> MAASRANDAPIVLLHGFTGWGREEMFGFKYWGGVRGDIEQWLNDNGYRTYTLAVGPLSSNWDRACEAYAQLVGGTVDYGAAHAAKHGHARFGRTYLGLLPELKRGGRIHIIAHSQGGQTARMLVSLLENGSQEEREYAKAHNVSLSPLFEGGHHFVLS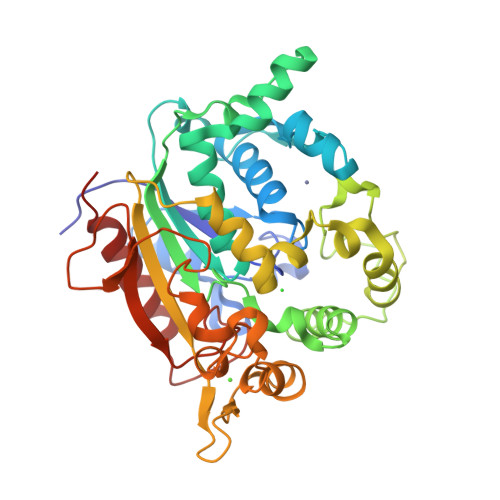VTTIATPHDGTTLVNMVDFTDRFFDLQKAVLEAAAVASNVPYTSQVYDFKLDQWGLRRQPGESFDHYFERLKRSPVWTSTDTARYDLSVSGAEKLNQWVQASPNTYYLSFATERTYRGALTGNYYPELGMNAFSAVVCAPFLGSYRNPTLGIDDRWLENDGIVNTVSMNGPKRGSSDRIVPYDGALKKGVWNDMGTYNVDHLEIIGVDPNPSFDIRAFYLRLAEQLASLQP> SDQEPLYPVQVSSADARLMVFDKTEGTWRLLCSSRSNARVAGLSCEEMGFLRALTHSELDVRTAGAAGTSGFFCVDEGRLPHTQRLLEVISVCDCPRGRFLAAICQDCGRRKLPVDRIVGGRDTSLGRWPWQVSLRYDGAHLCGGSLLSGDWVLTAAHCFPERNRVLSRWRVFAGAVAQ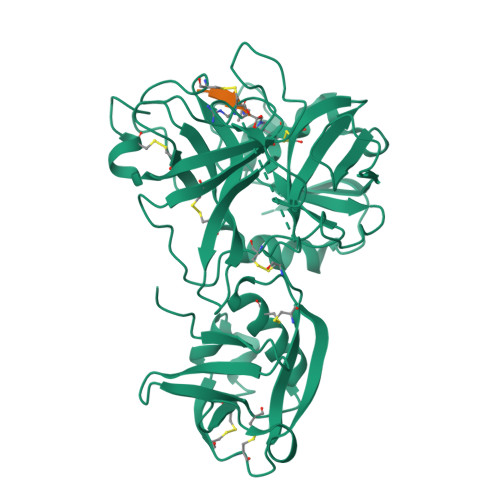ASPHGLQLGVQAVVYHGGYLPFRDPNSEENSNDIALVHLSSPLPLTEYIQPVCLPAAGQALVDGKICTVTGWGNTQYYGQQAGVLQEARVPIISNDVCNGADFYGNQIKPKMFCAGYPEGGIDACQGDSGGPFVCEDSISRTPRWRLCGIVSWGTGCALAQKPGVYTKVSDFREWIFQAIKTHSEASGMVTQL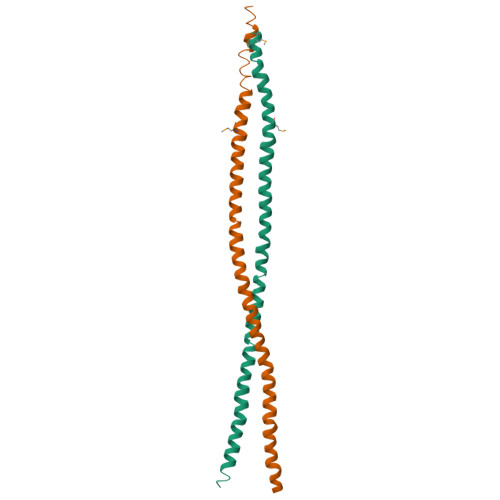>GPLGSLEEQLNKSLKTIASQKAAIENYNQLKEDYNTLKRELSDRDDEVKRLREDIAKENELRTKAEEEADKLNKEVEDLTASLFDEANNLVADARMEKYAIEILNKRLTEQLREKDMLLDTLTLQLKNLKKVMHS[20x]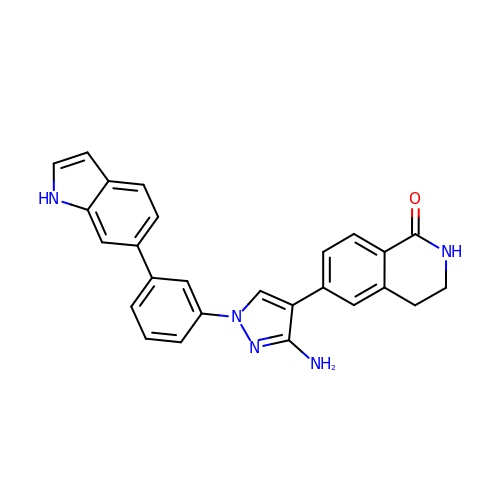6-{3-amino-1-[3-(1H-indol-6-yl)phenyl]-1H-pyrazol-4-yl}-3,4-dihydroisoquinolin-1(2H)-one | C26 H21 N5 O | ZTKOUSVWVUFWQC-UHFFFAOYSA-N>[3x]SMSKNNIFNKYPTIIHGEARGE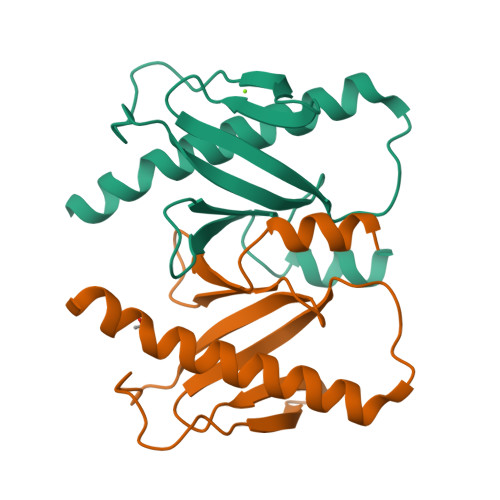NDEFVVHTRYPRFLARKSFDDNFTGEMPAKPVNGELGQIGEPRRLAYDSRLGLWLSDFIMLDNNKPKNMEDWLGQLKAACDRIAADDLMLNEDAADLEGWDD> MSSTVISRKRRNSTVTEPDSSGETRKQKKSRSDEKSSSSKDGDPQLEFKVLQGYRDLESEMHKGRAQVTRTGDIGVAMDNLNAVDSLFNKVIGIKNNGLFAHDARAMVSISELAQISVRNLKFDDSRSMVNLENIVNSLKRYMLKEHFKLNNIAENRNDLTLAADEQSAADQQEESDGDIDRTPDDNHTDKATSSFKATSMRHSYLQQFSHYNEFSQFNWFRIGALYNTISKNAPITDHLMGPLSIEKKPRVLTQRRRNNDQVGEKITAEKITQHSLNSTQQETTPEQVKKCFKKLSKKLGPEGSINLFKFIIDPNSFSRSIENLFYTSFLIKEGKLLMEHDEEGLPTIKIKQSISHTDSRSKEIERQRRRAAHQNHIIFQMDMPTWRKLIKKYNITSPFLD;> MEVHEEQVSAPVTGDATAKYLLQYILSARGICHENALILALMRLETDASTLNTEWSIQQWVDKLNDYINAINVKLNLLGYKIIRINHGIGRNAVTLKAKQNFESFEDNTAIRAHNNDYAVLQSIVLPESNRFFVYVNLASTEETKLATRFNQNEIEFMKWAIEQFMISGETIVEGPALETSIIVKEVNRILVAATGDSNLAKWRKFSTFTVGSTNLFQFQELTATDIEDLLLRLCELKWFYRTQEGKFGIDLRCIAELEEYLTSMYNLNTCQNCHKLAIQGVRCGNESCREENEETGENSLSQIWHVDCFKHYITHVSKNCDRCGSSLITEGVYVI;> MSSIDNDSDVDLTEDLAVAKIVKENPVARKMVRYILSRGESQNSIITRNKLQSVIHEAAREENIAKPSFSKMFMDINAILYNVYGFELQGLPSKNNMNAGGNGSNSNTNKSMPEPLGHRAQKFILLNNVPHSKNFDDFKILQSAHTYEELIVTGEYIGDDIASGTSNTLESKLSTDRDLVYKGVLSVILCIVFFSKNNILHQELIKFLETFGIPSDGSKIAILNITIEDLIKSLEKREYIVRLEEKSDTDGEVISYRIGR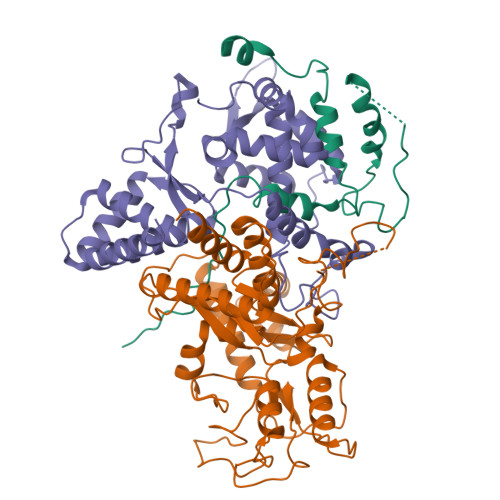RTQAELGLESLEKLVQEIMGLEKEQTKSLHDDIIKSIGDSYSI> MFKTE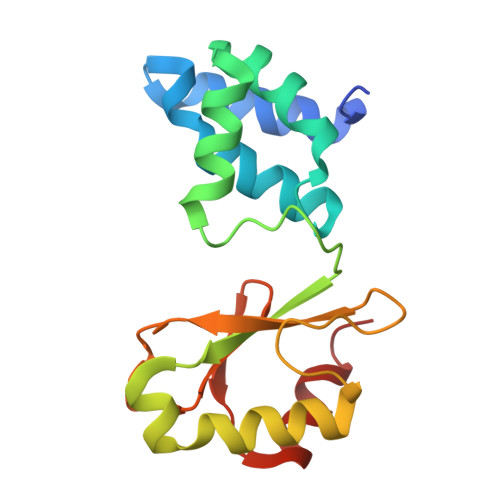FEFPEELKTKLQEHINYFPKKRQAILLCLHEIQNYYGYIPPESLKPLADMLELPLNHVEGVVAFYDMFDREDKAKYRIRVCVSIVCHLMGTNKLLKALENILGIKPGEVTPDGKFKIVPVQCLDACSEAPVFMVNDDEYKFESEVQLNEILSRYT>[2x]GSHMETVAAIKTLIQQLAQSTDQFGRAEINDALRELQYSLETPFDTVMRMSLDTCQVAVARIGSDLGLFKHLSQCASPQSAEELADHLGCGRELMSRL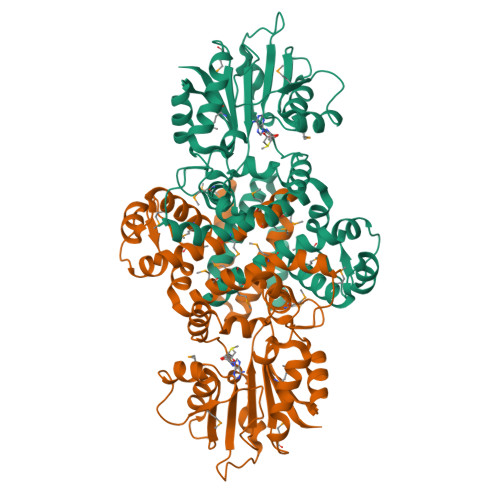LRYMASVRMVQQTDDIKYISSNITQTLAVPGLEAGMRHAFENLWPVLMALPDFLAERKYPDIVDAKDTAFQKAFNTDQDCFHWLATQPTRIANFKVLLTDERTPNFLSTFPLEKELGSWSAEPEKALFVDIGGGMGHACIRLREKYPNQPGRVILQDLPPVLQAAQATLPLSGIESMPHNFHTPQPVQGAKFYFLRLILRDFPDHQALEILQNIVPAMDAESRIVIDDGVPPEKGARWAETGTDICIMSALGSKERTQRQWEELAAKAGLQLQALYQYTWPVVNAAMVFSLQ> APLVHHHHHHALDENLYFQGALADVSRPPHARKTGGSSPETKYDQPPKCDISGKEAISALSRAKSKHCRQEIGETYCRHKLGLLMPEKVTRFCPLEGKANKNVQWDEDSVEYMPANPVRIAFVLVVHGRASRQLQRMFKAIYHKDHFYYIHVDKRSNYLHRQVLQVSRQYSNVRVTPWRMATIWGGASLLSTYLQSMRDLLEMTDWPWDFFINLSAADYPIRTNDQLVAFLSRYRDMNFLKSHGRDNARFIRKQGLDRLFLECDAHMWRLGDRRIPEGIAVDGGSDWFLLNRRFVEYVTFSTDDLVTKMKQFYSYTLLPAESFFHTVLENSPHCDTMVDNNLRITNWNRKLGCKCQYKHIVDWCGCSPNDFKPQDFHRFQQTARPTFFARKFEAVVNQEIIGQ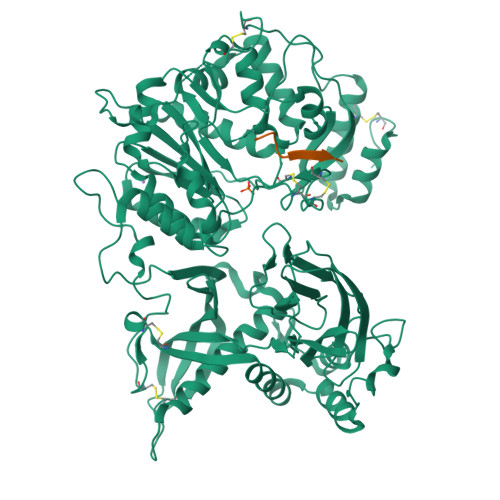LDYYLYGNYPAGTPGLRSYWENVYDEPDGIHSLSDVTLTLYHSFARLGLRRAETSLHTDGENSCRYYPMGHPASVHLYFLADRFQGFLIKHHATNLAVSKLETLETWVMPKKVFKIASPPSDFGRLQFSEVGTDWDAKERLFRNFGGLLGPMDEPVGMQKWGKGPNVTVTVIWVDPVNVIAATYDILIESTAEFTHYKPPLNLPLRPGVWTVKILHHWVPVAETKFLVAPLTFSNRQPIKPEEALKLHNGPLRNAYMEQSFQSLNPVLSLPINPAQVEQARRNAASTGTALEGWLDSLVGGMWTAMDICATGPTACPVMQTCSQTAWSSFSPDPKSELGAVKPDGRLR;> QEEEGSGVGQGG>PGMDSLPNPYLQSVSLTVCYMVKIKANLLSPFGKNPELQVDFGTGTGQGGDIPFRFWYCDGIVVMNTLKDGSWGKEQKLHTEAFVPGQPFELQFLVLENEYQVFVNNKPICQFAHRLPLQSVKMLDVRGDIVLTSVDTL[8x]

Galectins are proteins that specifically bind to β-galactoside sugars. In animals, for instance, nematode larvae induce increased expression of galectin-11, which is produced by epithelial cells and secreted into the gut lumen, coinciding with an eosinophil-biased inflammatory response characteristically associated with larval infection(s). As a functional analogue of galectin-1, galectin-11 is proposed to cross-link glycans in mucus to form a physical barrier against the parasite(s), as part of a pronounced inflammatory response. The crystal structure of LGALS-11 has a folding pattern that is similar to prototype galectins-1, -2 and -10, suggesting a relatively conserved ligand-binding activity.

First, we solved the crystal structure of LGALS-11 in apo form to 2.0 Å complexed with β-D-galactose at 2.4 Å. LGALS-11 forms a homodimer via hydrogen bonds between residues L9 and S11 of monomers (i), and is inferred to have two unique cell attachment sites (called LDV and RGD) for integrin binding (ii). The LGALS-11 crystal structure enabled the localisation of the precise residue variation in the dimer interface connecting β-strands of two monomers, the glycan-binding groove and the putative integrin-binding site. The residue substitution from a hydrophobic residue (leucine) in isoform 1 to a polar or charged residue (glutamine) in isoform 2 is likely to hinder dimer formation, and energetically favour contact with water rather than the complementary polar (serine) residue (S11) to form a homodimer. Through sedimentation velocity studies, we confirmed that the residue substitution in the dimer interface affects the homodimers and subsequent oligomerisation of LGALS-11. The c(s) distributions at concentrations of 0.10, 0.30 and 0.90 mg/ml showed that isoform 1 is represented by a tetramer at all concentrations tested (sedimentation coefficient: 4.0 S), whereas isoform 2 is in a monomer–dimer equilibrium (sedimentation coefficients: 1.64 S and 2.5 S, respectively). To verify the tetrameric organisation of isoform 1, we then mutated residues L9 and S11 to alanine, produced a recombinant dimerisation mutant (DI-m) protein and assessed the sedimentation velocity of this protein. This DI-m protein exists as a monomer–dimer equilibrium (sedimentation coefficients: 1.1 S (monomer) and 1.7 S (dimer), respectively), similar to isoform 2. In addition, we demonstrated that only the homotetrameric form of LGALS-11 inhibits H. contortus larval development, and causes direct damage to the surface of the L4, an indication of loss of viability and death. No anti-parasitic activity was detected for isoform 2 or the dimerisation interface (DI-m) or carbohydrate recognition (CRD-m) mutant, indicating that extended oligomerisation or lattice formation via self-dimerisation and glycan recognition properties is critical for the anti-parasitic effect.>[4x]MTTTAPPQTVPTKTVPSKTVASIRWLAAPTSWSWVEQANAHPMEVLIDHAHCERKAAGAAVQ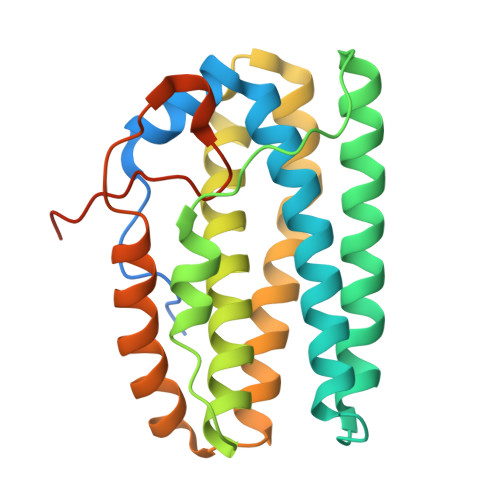MMFRYLCEPGLGEALSPLAREELEHFEQVLALIKARGRYLEPLPSPGYGADLARQIRKGEPQRMLDSFLVAGLIEARSHERMALLAEHSPDPQLRELYSDLLASEARHFGLYWVLCEQRYPRELIVERLEVLALAEVKALEGALTRPEDVRMHSCGVDVTQISSQISGSHHHHHH>[2x]ESYLSPAQSVKPKINTEEKLPREKLNPPTPSIYLESKRDAFSPVLLQFCTDPRNPITVIRGLAGSLRLNLGLFSTKTLVEASGEHTVEVRTQVQQPSDENWDLTGTRQIWPCESSRSHTTIAKYAQYQASSFQESLQEELEVLFQGPTKAARKSAPATGGGSSGSHHIIKFGTNIDLSDAKRWKPQLQELLKLPAFMRVTSTG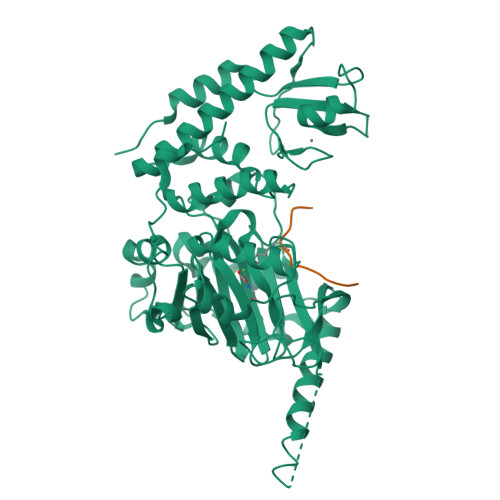NMLSHVGHTILGMNTVQLYMKVPGSRTPGHQENNNFCSVNINIGPGDCEWFAVHEHYWETISAFCDRHGVDYLTGSWWPILDDLYASNIPVYRFVQRPGDLVWINAGTVHWVQATGWCNNIAWNVGPLTAYQYQLALERYEWNEVKNVKSIVPMIHVSWNVARTVKISDPDLFKMIKFCLLQSMKHCQVQRESLVRAGKKIAYQGRVKDEPAYYCNECDVEVFNILFVTSENGSRNTYLVHCEGCARRRSAGLQGVVVLEQYRTEELAQAYDAFTLAPASTSR;>[2x]AARKSAPATGG>[20x]MSPLRPQNYLFGCELKADKDYHFKVDNDENEHQ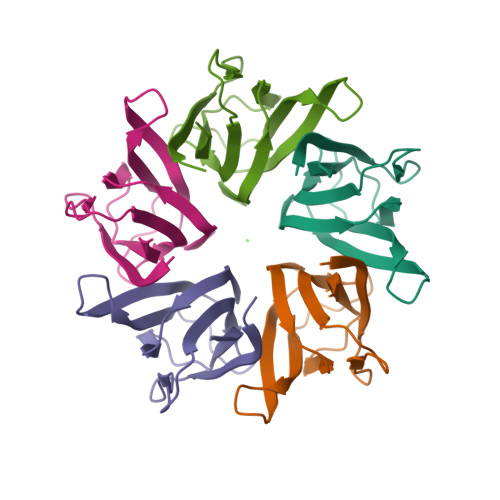LSLRTVSLGAGAKDELHIVEAEAMNYEGSPIKVTLATLKMSVQPTVSLGGFEITPPVVLRLKCGSGPVHISGQHLVAVEEDAE Aromatic residues cluster in the core of folded proteins, where they stabilize the structure through multiple interactions. NMR studies in the 1970s demonstrated that aromatic side chains can undergo ring flips—that is, 180° rotations of the χ2 dihedral angle (Cβ–Cγ axis)—even when engaged in stabilizing interactions in the hydrophobic core. Here we capture ring flipping events of a buried tyrosine residue in the SH3 domain of the JNK-interacting protein 1 (JIP1). Our data therefore suggest that the conformation of the aromatic ring at position 526 is determined by steric interactions dictated by the size of the surrounding amino acids.

We therefore hypothesized that SH3 domains of group 1 have eclipsed conformations, whereas group 2 have staggered conformations. To test our hypothesis, we determined two crystal structures of SH3 domains of the scaffold protein POSH (‘plenty of SH3 domains’), for which the first SH3 domain belongs to group 2 and the fourth SH3 domain belongs to group 1. POSH-SH3-4 shows a similar structure to JIP1-SH3, with an eclipsed conformation of the corresponding phenylalanine residue (F867) stabilized by CH–π interactions from V858 (position 517), K861 (position 520) and G882 (position 541), and by π–π interactions with H834 (position 493).

> GRRVVCERHRVVVSYPPQSEAELELKEGDIVFVHKKREDGWFKGTLQRNGKTGLFPGSFVENI>MTDNNKYRDVEIRAPRGNKLTAKSWLTEAPLRMLMNNLDPQVAENPKELVVYGGIGRAARNWECYDKIVETLTRLEDDETLLVQSGKPVGVFKTHSNAPRVLIANSNLVPHWANWEHFNELDAKGLAMYGQMTAGSWIYIGSQGIVQGTYETFVEAGRQHYGGSLKGKWVLTAGLGGMGGAQPLAATLAGACSLNIESQQSRIDFRLETRYVDEQATDLDDALVRIAKYTAEGKAISIALHGNAAEILPELVKRGVRPDMVTDQTSAHDPLNGYLPIGWTWEQYRDRAQTI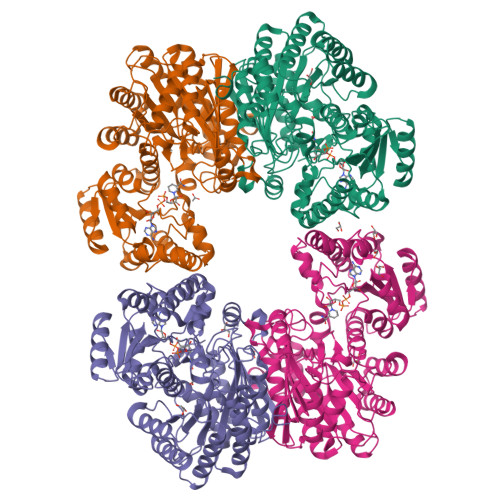PAAVVKAAKASMAVHVQAMLDFQKQGVPTFDYGNNIRQMAKEEGVANAFDFPGFVPAYIRPLFCRGVGPFRWAALSGEAEDIYKTDAKVKELIPDDAHLHRWLDMARERISFQGLPARICWVGLGLRAKLGLAFNEMVRSGELSAPVVIGRDHLDSGSVSSPNRETEAMRDGSDAVSDWPLLNALLNTAGGATWVSLHHGGGVGMGFSQHSGMVIVCDGTDEAAERIARVLTNDPGTGVMRHADAGYDIAIDCAKEQGLDLPMITG[4x]> MAKQYDSVECPFCDEVSKYEKLAKIGQGTFGEVFKARHRKTGQKVALKKVLMENEKEGFPITALREIKILQLLKHENVVNLIEICRTKASPYNRCKGSIYLVFDFCEHDLAGLLSNVLVKFTLSEIKRVMQMLLNGLYYIHRNKILHRDMKAANVLITRDGVLKLADFGLARAFSLAKNSQPNRYTNRVVTLWYRPPELLLGERDYGPPIDLWGAGCIMAEMWTRSPIMQGNTEQHQLALISQLCGSITPEVWPNVDNYELY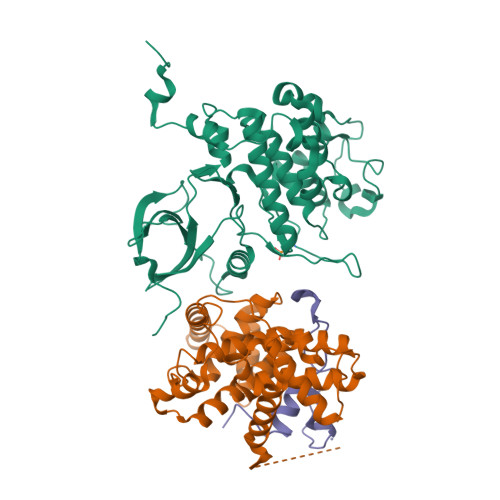EKLELVKGQKRKVKDRLKAYVRDPYALDLIDKLLVLDPAQRIDSDDALNHDFFWSDPMPSDLKGMLSTHLTSMFEYLAPPRRKHHHHHH;> MEGERKNNNKRWYFTREQLENSPSRRFGVDPDKELSYRQQAANLLQDMGQRLNVSQLTINTAIVYMHRFYMIQSFTQFPGNSVAPAALFLAAKVEEQPKKLEHVIKVAHTCLHPQESLPDTRSEAYLQQVQDLVILESIILQTLGFELTIDHPHTHVVKCTQLVRASKDLAQTSYFMATNSLHLTTFSLQYTPPVVACVCIHLACKWSNWEIPVSTDGKHWWEYVDATVTLELLDELTHEFLQILEKTPNRLKRIWNWRACEAAKK;> MEPVDPRLEPWKHPGSQPKTACTNCYCKKCCFHCQVCFITKALGISYGRKKRRQRRRAHQNSQTHQASLSKQPTSQSRGDPTGPKE(3~{S},7~{R},10~{R},13~{S})-4-[(3~{S},6~{R},8~{a}~{S})-1'-[(2~{S})-2-acetamido-3-(2-chlorophenyl)propanoyl]-5-oxidanylidene-spiro[1,2,3,8~{a}-tetrahydroindolizine-6,2'-pyrrolidine]-3-yl]carbonyl-2-oxidanylidene-1,4-diazatricyclo[8.3.0.0^{3,7}]tridec-8-ene-13-carboxylic 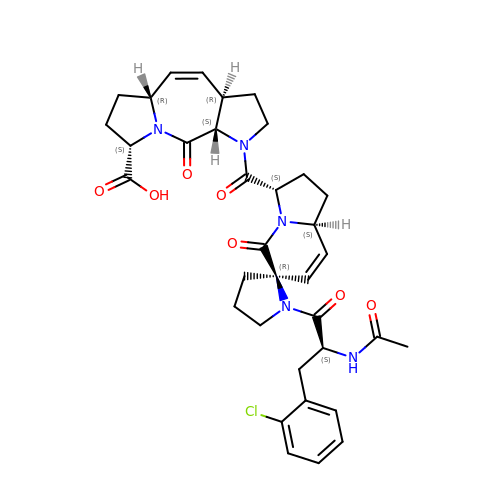acid | C35 H40 Cl N5 O7 | AYDUPBNKBXOHLZ-QHVDBZGRSA-N> TRSFYNDGHLNGWDYVRKENQGTVSEVSNVVFKGTSALKMTQTYTPGYTGRYHSEVDHNRGYQRGEEQFYGFAFRLSEDWQFQPQSYNIAQFIANRPGAGCGGDDWMPSTMIWIQNNQLYSRYVNGHYRQPNCGRNIVTRPNLATVSAGAWHRVVLQIKWASDNTGYFKIWFDGAKVHEEYNVATTVDDDSVFQFRVGLYA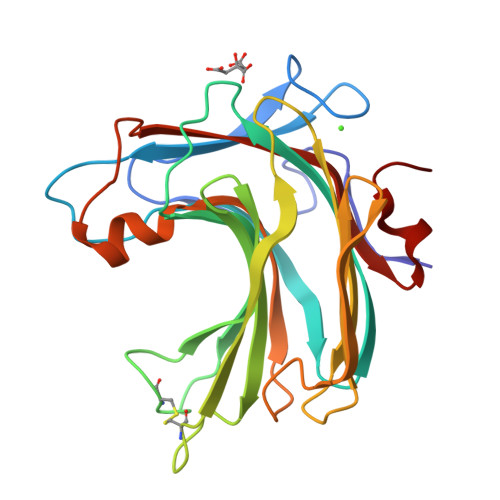NSWHDDGHMTGTQGFRQVWYDEVAVGTTFADVDPDQA>MRVLLIHSDYIEYEVKDKALKNPEPISEDMKRGRMEEVLVAFISVEKVDEKNPEEVSLKAIEEISKVAEQVKAENVFVYPFAHLSSELAKPSVAMDILNRVYQGLKERGFNVGKAPFGYYMAFKISCKGHPLAELSRTIVPEEARVE[2x]

We have been interested in a D-aminoacyl-tRNA deacylase (DTD) fold that is present across the domains of life in two different functional contexts: as an N-terminal editing domain (NTD) of archaeal ThrRS, which specifically removes non-cognate L-serine mischarged on tRNAThr, and as a freestanding ‘chiral proofreading' enzyme, which removes D-amino acids from tRNAs in bacteria and eukaryotes. Both share a striking structural and mechanistic similarity highlighting a common ancestry. Here we show, with the help of structural, biochemical and biophysical studies from three distant organisms, that the substrate specificity in this domain is determined by a differential remodelling of the catalytic centre at the RNA–protein interface rather than just the presence or absence of catalytic water as previously proposed. While demonstrating that the tRNA provides the catalytic group, we show that the side chains within the recognition site are dispensable for the proofreading function, suggesting a primordial mode of protein- or peptide scaffold-based enzymatic activity evolved alongside that of RNA.

On the other hand, the Lys to Met mutant, although showed partial activity against L-Ser-(Ec)tRNAThr in our earlier work, in subsequent studies with not only PabNTD K121M but also the corresponding K116M and K122M mutants of ApNTD and MjNTD with multiple batches of protein showed a severely compromised activity, suggesting a crucial role of this residue in enzyme function. However, a direct role of Lys in catalysis is still highly unlikely considering that this position is naturally occupied by a Met in the structural homologue DTD. We solved the crystal structure of K121M mutant of PabNTD and K116M mutant of ApNTD with L-Ser3AA and L-Thr3AA to investigate the structural basis of the observed loss of activity. A significant repositioning of the crucial catalytic water was observed upon mutation of the polar Lys side chain to the non-polar Met side chain, which is present in DTD. This provides a clear structural basis for the loss of function in this mutant, despite its high binding affinity for the substrate. Therefore, we show that Lys plays a crucial role in positioning the water molecule for catalysis rather than acting as a nucleophile.> MGSDKIHHHHHHENLYFQGYRPLFDKDLSNADYDSSVWTFKNGILTATADQSIWTKVQYENFILDLEFKTDVNTNSGVVIYCTDKGNWIPSSIEIQIADDHHPEWQSYPEYWRCGSIYGHKGANEQLVVKKPGEWNRMI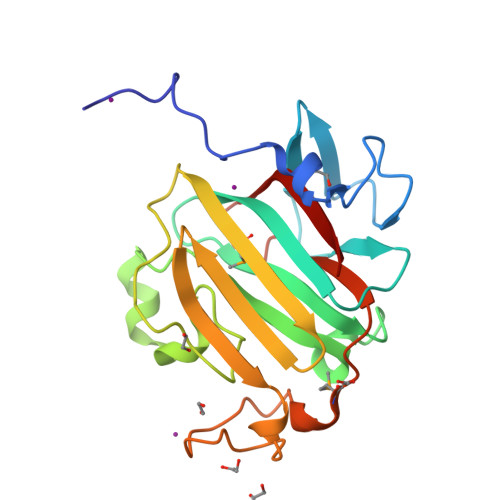ITAKGQQIDIELNGKHIVSANLADWTSGTTNPDGTEIPEWLPIPYANMPTKGYIGLQGKHGESNIWFRNIQLKQL> E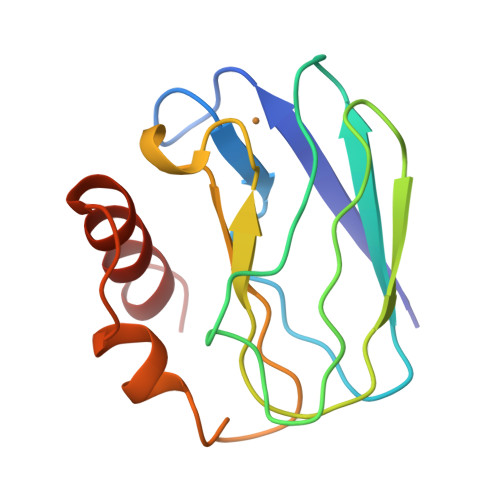NIEVHMLNKGAEGAMVFEPAYIKANPGDTVTFIPVDKGHNVESIKDMIPEGAEKFKSKINENYVLTVTQPGAYLVKCTAHYAMGMIALIAVGDSPANLDQIVSAKKPKIVQERLEKVIASAK Transcription activator-like (TAL) effectors specifically bind to double stranded (ds) DNA through a central domain of tandem repeats. Each TAL effector (TALE) repeat comprises 33–35 amino acids and recognizes one specific DNA base through a highly variable residue at a fixed position in the repeat. The crystal structures of TAL effector (TALE) proteins bound to their respective target DNAs have revealed that the residue at position 13 is the only one directly involved in DNA base recognition, whereas the 12th residue stabilizes the proper loop conformation. dHax3, an engineered TALE protein, proved to be a useful scaffold for structural characterizations. We then present fifteen crystal structures of engineered dHax3 variants in complex with target DNA molecules, which elucidate the structural basis for the recognition of bases adenine (A) and guanine (G) by reported or uncharacterized TALE codes.

The structural observation suggests that Ile34 may not be a major contributor to the affinity of DNA binding by TALE repeats, consistent with the classification of NI as a “weak” TALE code. It also insinuates that base A may “tolerate” a wide range of amino acids at position 34 of a TALE repeat when there is no steric clash. To test this speculation, we generated dHax3 variants with the 34th residue on repeat 7 substituted with different amino acids. In total, we obtained nine high-quality structures that elucidate the accommodation of base A by Leu, Met, Cys, Pro, Trp, His, Thr, Asn, and Glu at the 34th position. Among these, the hydrophobic residues Leu, Met, Cys, and Pro all adopt conformations that do not clash with base A. As what happens to Ile34, there is no specific coordination found between these hydrophobic residues and base A. Trp, Thr, and His, in spite of the presence of polar groups, do not form H-bond with base A. They also appear to adopt conformations that simply avoid steric clash. These residues may all represent weak code, if they are used for base recognition.

>[2x]MQWSGARALEALLTVAGELRGPPLQLDTGQLLKIAKRGGVTAVEAVHAWRNALTGAPLNLTPEQVVAIASHDGGKQALETVQRLLPVLCQAHGLTPQQVVAIASHDGGKQALETVQRLLPVLCQAHGLTPEQVVAIASHDGGKQALETVQALLPVLCQAHGLTPEQVVAIASNGGGKQALETVQRLLPVLCQAHGLTPQQVVAIASNGGGKQALETVQRLLPVLCQAHGLTPQQVVAIASNGGGKQALETVQRLLPVLCQAHGLTPQQVVAIASNMGGKQALETVQRLLPVLCQAHGLTPQQVVAIASNGGGKQALETVQRLLPVLCQAHGLTPQQVVAIASHDGGKQALETVQRLLPVLCQAHGLTPEQVVAIASNGGGKQALETVQRLLPVLCQAHGLTPEQVVAIASHDGGKQALETVQRLLPVLCQAHGLTPQQVVAIASNGGGRPALESIVAQLSRPDPALAALTNDHLVALACLGGRPALDAVKKLEHHHHHH> MAHHHHHHHHHHSGRAEDKSKRDSIEMSMKGCQTNNGFVHNEDILEQTPDPGSSTDNLKHSTRGILGSQEPDFKGVQPYAGMPKEVLFQFSGQARYRIPREILFWLTVASVLVLIAATIAIIALSPKCLDWWQEGPMYQIYPRSFKDSNKDGNGDLKGIQDKLDYITALNIKTVWITSFYKSSLKDFRYGVEDFREVDPIFGTMEDFENLVAAIHDKGLKLIIDFIPNHTSDKHIWFQLSRTRTGKYTDYYIWHDCTHENGKTIPPNNWLSVYGNSSWHFDEVRNQCYFHQFMKEQPDLNFRNPDVQEEIKEILRFWLTKGVDGFSLDAVKFLLEAKHLRDEIQVNKTQIPDTVTQYSELYHDFTTTQVGMHDIVRSFRQTMDQYSTEPGRYRFMGTEAYAESIDRTVMYYGLPFIQEADFPFNNYLSMLDTVSGNSVYEVITSWMENMPEGKWPNWMIGGPDSSRLTSRLGNQYVNVMNMLLFTLPGTPITYYGEEIGMGNIVAANLNESYDINTLRSKSPMQWDNSSNAGFSEASNTWLPTNSDYHTVNVDVQKTQPRSALKLYQDLSLLHANELLLNRGWFCHLRNDSHYVVYTRELDGIDRIFIVVLNFGESTLLNLHNMISGLPAKMRIRLSTNSADKGSKVD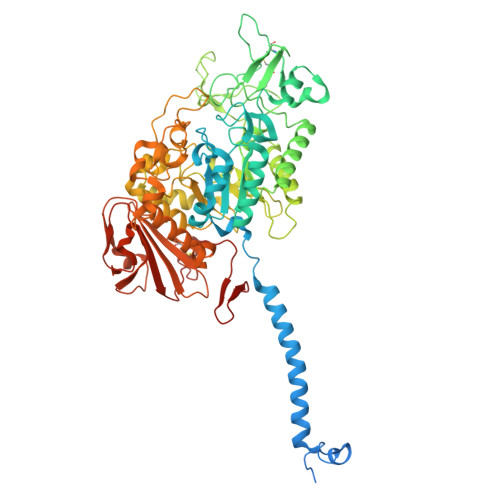TSGIFLDKGEGLIFEHNTKNLLHRQTAFRDRCFVSNRACYSSVLNILYTSC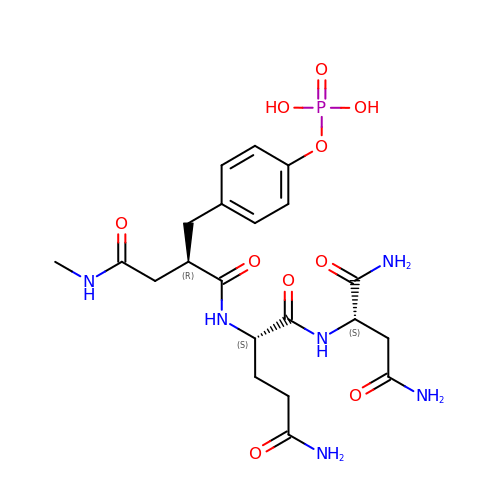N~2~-{(2R)-4-(methylamino)-4-oxo-2-[4-(phosphonooxy)benzyl]butanoyl}-L-glutaminyl-L-aspartamide | C21 H31 N6 O10 P | KWOJJSIJYPOAJI-SNPRPXQTSA-N> RYNDYKLDFRRQQMQDFFLAHKDEEWFRSKYHPDEVGKRRQEARGALQNRLRVFLSLMETGWF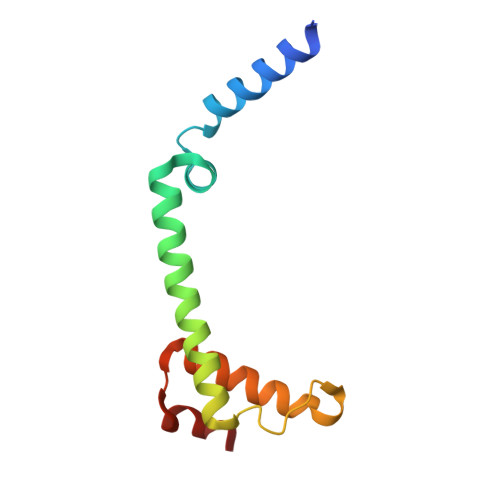DNLLLDIDKADAIVKMLDAAVIKMEGGTENDLRILEQ>[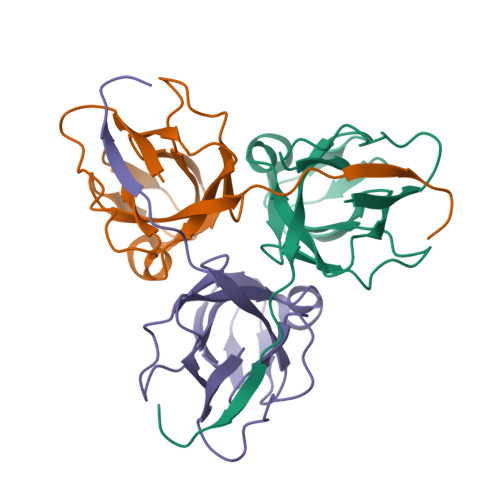3x]MQIKIKYLDETQTRINKMEQGDWIDLRAAEDVAIKKDEFKLVPLGVAMELPEGYEAHVVPRSSTYKNFGVIQTNSMGVIDESYKGDNDFWFFPAYALRDTKIKKGDRICQFRIMKKMPAVDLIEVDRLGNGDRGGHGSTGTK>TNRLQGKVALVTGGASGVGLEVVKLLLGEGAKVAFSDINEAAGQQLAAELGERSMFVRHDVSSEADWTLVMAAVQRRLGTLNVLVNNAGILLPGDMETGRLEDFSRLLKINTESVFIGCQQGIAAMKETGGSIINMASVSSWLPIEQYAGYSASKAAVSALTRAAALSCRKQGY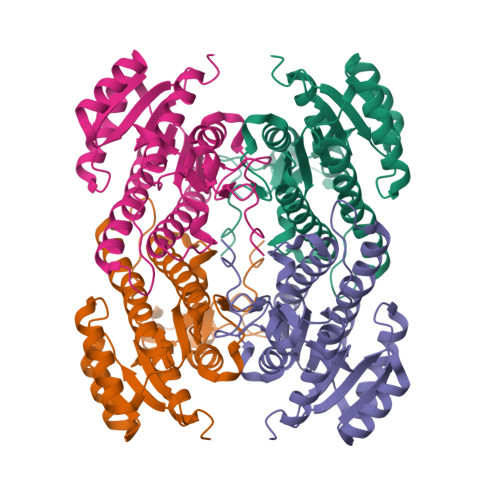AIRVNSIHPDGIYTPMMQASLPKGVSKEMVLHDPKLNRAGRAYMPERIAQLVLFLASDESSVMSGSELHADNSILGMGL[4x]> HHHHHHHSEMTPREIVSELDKHIIGQDNAKRSVAIALRNRWRRMQLNEELRHEVTPKNILMIGPTGVGKTEIARRLAKLANAPFIKVEATKFTEVGYVGKEVDSIIRDLTDAAVKMVRVQAIEKNRYRAEELAEERILDVLIPPAKNNWGQTEQQQEPSAARQAFRKKLREGQLDDKEIEIDLAAAPMGVEIMAPPGMEEMTSQLQSMFQNLGGQKQKARKLKIKDAMKLLIEEEAAKLVNPEELKQDAIDAVEQHGIVFIDEIDKICKRGESSGPDVS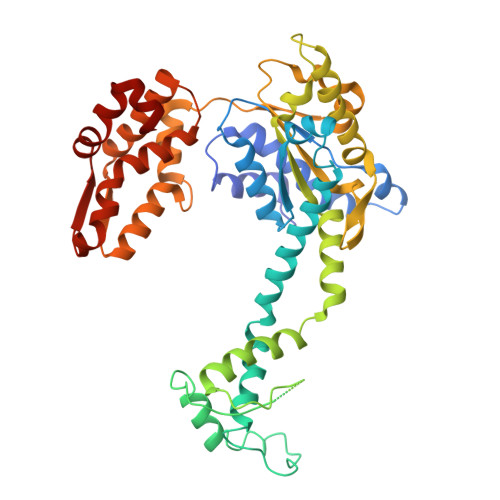REGVQRDLLPLVEGCTVSTKHGMVKTDHILFIASGAFQIAKPSDLIPELQGRLPIRVELQALTTSDFERILTEPNASITVQYKALMATEGVNIEFTDSGIKRIAEAAWQVNESTENIGARRLHTVLERLMEEISYDASDLSGQNITIDADYVSKHLDALVADEDLSRFIL> MIKIIKNAKVFSPEYIGKKDVIFYHKVIHVGEGVNTSVLPFEHEIYDANGLLLLPGLIDPHVHITGGGGEGGFETRTPELKISDCIRSGVTTVVGCLGTDGITRSLENLYAKAKSLESEGLNTFIYTGSYRVPPVTFTGSIMRDIVLIDKVIGVGEIAISDHRSSQPTLEEILRIVADIRVGGMISGKAGIVNFHVGSGKRGIEYLFDIIEKTEIPIQHLYPTHMSRSRKLFEQGLEFAKRGGTIDLTALQPKDAEFVRAEFTTIDAICEAYENGLLDNVTISSDGQGSLPKFDDNGNFVGLDVGSVSAVWYTIRKVLEKGLPLAEVLKISTTNPARVFKLNKGKIAKGQ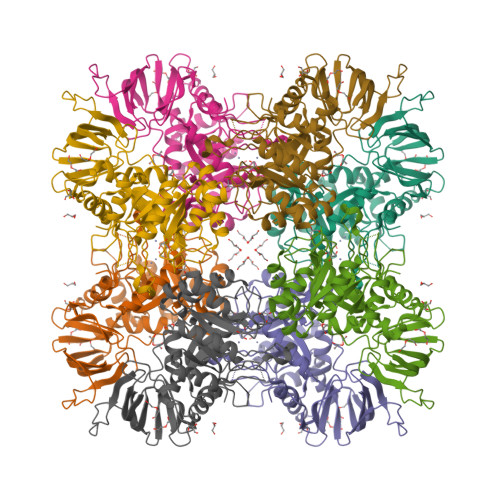DADFILVDEQSFEIVSVISKGEFLMKDGVMKNLNFEF(2E)-2-ethylidene-4-hydroxy-5-methylfuran-3(2H)-one | C7 H8 O3 | 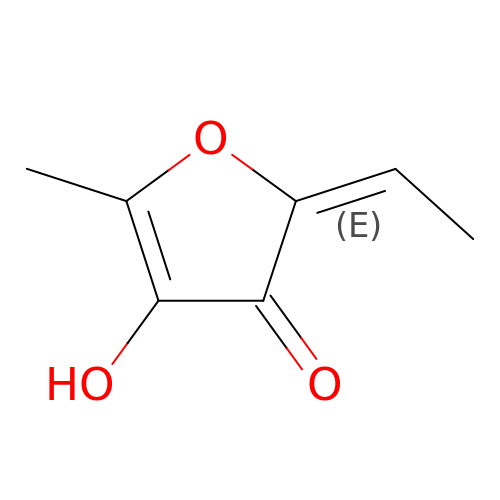CWXWDRXNERDGHE-HWKANZROSA-N>[4x]SNAMDKNIIIGAMTALITPFKNGKVDEQSYARLIKRQIENGIDAVVPVGTTGESATLTHEEHRTCIEIAVETCKG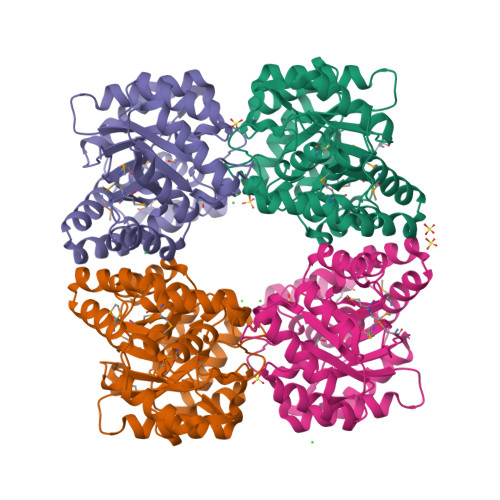TKVKVLAGAGSNATHEAVGLAKFAKEHGADGILSVAPYYNKPTQQGLYEHYKAIAQSVDIPVLLYNVPGRTGCEISTDTIIKLFRDCENIYGVKEASGNIDKCVDLLAHEPRMMLISGEDAINYPILSNGGKGVISVTSNLLPDMISALTHFALDENYKEAKKINDELYNINKILFCESNPIPIKTAMYLAGLIESLEFRLPLCSPSKENFAKIEEVMKKYKIKGF>[2x]GFKQDIATIRGDLRTYAQDIFLAFLNKYPDERRYFKNYVGKSDQELKSMAKFGDHTEKWFNLMMEVADRATDCVPLASDANTLV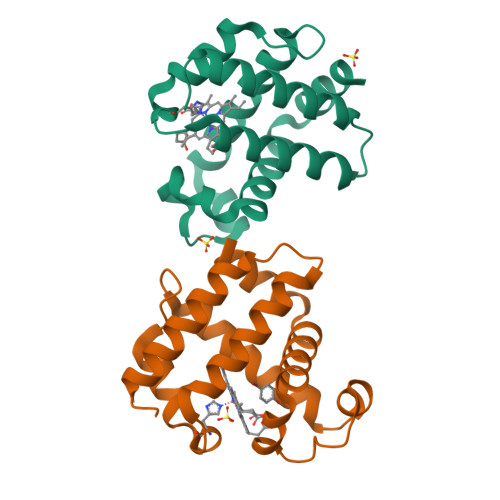QMKQHSSLTTGNFEKLFVALVEYMRASGQSFDSQSWDRFGKNLVSALSSAGMK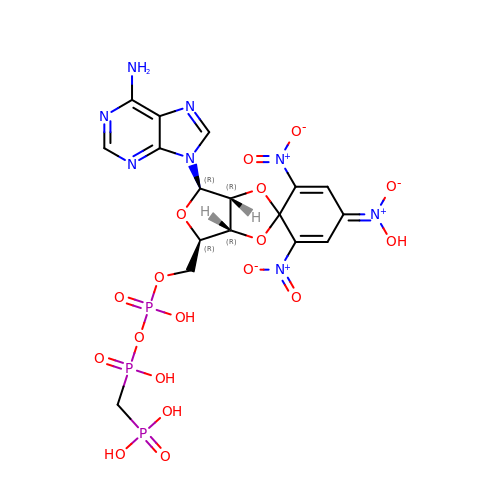Spiro(2,4,6-trinitrobenzene[1,2a]-O2',O3'-methylene-adenosine (beta,gamma-methylene)triphosphate | C17 H19 N8 O18 P3 | WOUJMFLAWZHYLK-KWDXPJCYSA-N> MEAEPPLYPMAGAAGPQGDEDLLGVPDGPEAPLDELVGAYPNYNEEEEERRYYRRKRLGVLKNVLAASAGGMLTYGVYLGLLQMQLILHYDETYREVKYGNMGLPDIDSKMLMGINVTPIAALLYTPVLIRFFGTKWMMFLAVGIYALFVSTNYWERYYTLVPSAVALGMAIVPLWASMGNYITRMAQKYHEYSHYKEQDGQGMKQRPPRGSHA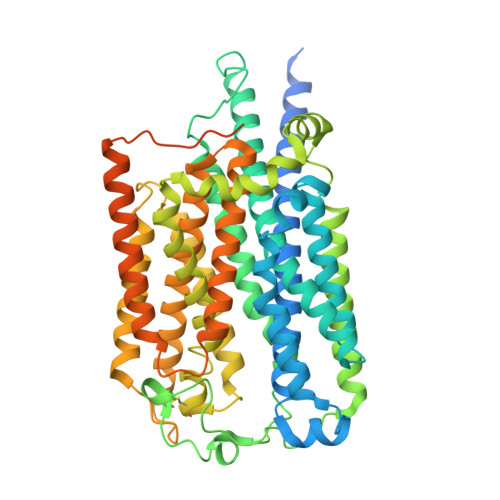PYLLVFQAIFYSFFHLSFACAQLPMIYFLNHYLYDLNHTLYNVQSCGTNSHGILSGFNKTVLRTLPRSGNLIVVESVLMAVAFLAMLLVLGLCGAAYRPTEEIDLRSVGWGNIFQLPFKHVRDYRLRHLVPFFIYSGFEVLFACTGIALGYGVCSVGLERLAYLLVAYSLGASAASLLGLLGLWLPRPVPLVAGAGVHLLLTFILFFWAPVPRVLQHSWILYVAAALWGVGSALNKTGLSTLLGILYEDKERQDFIFTIYHWWQAVAIFTVYLGSSLHMKAKLAVLLVTLVAAAVSYLRMEQKLRRGVAPRQPRIPRPQHKVRGYRYLEEDNSDESDAEGEHGDGAEEEAPPAGPRPGPEPAGLGRRPCPYEQAQGGDGPEEQ>NEDMPVERILEAELAVEPKTETYVEANMGLNPSSPNDPVTNICQAADKQLFTLVEWAKRI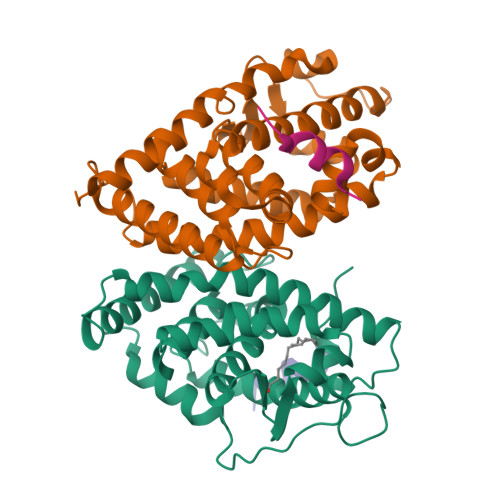PHFSELPLDDQVILLRAGWNELLIASFSHRSIAVKDGILLATGLHVHRNSAHSAGVGAIFDRVLTELVSKMRDMQMDKTELGCLRAIVLFNPDSKGLSNPAEVEALREKVYASLEAYCKHKYPEQPGRFAKLLLRLPALRSIGLKCLEHLFFFKLIGDTPIDTFLMEMLEAPHQMT[2x];>[2x]PVQLSKEQEELIRTLLGAHTRHMGTMFEQFVQFRPPAHLFIHHQPLPTLAPVLPLVTHFADINTFMVLQVIKFTKDLPVFRSLPIEDQISLLKGAAVEICHIVLNTTFCLQTQNFLCGPLRYTIEDGARVGFQVEFLELLFHFHGTLRKLQLQEPEYVLLAAMALFSPDRPGVTQRDEIDQLQEEMALTLQSYIKGQQRRPRDRFLYAKLLGLLAELRSINEAYGYQIQHIQGLSAMMPLLQEICS;>[4x]ERHKILHRLLQEG> MGKYFGTDGVRGVANSELTPELAFKVGRFGGYVLTKDKQRPKVLIGRDTRISGHMLEGALVAGLLSIGAEVMRLGVISTPGVSYLTKAMDAEAGVMISASHNPVQDNGIKFFGGDGFKLSDEQEAEIERLMDEPEDKLPRPVGADLGLVNDYFEGGQKYLQFLKQTADEDFTGIHVALDCANGATSSLATHLFADLDADVSTMGTSPNGLNINDGVGSTHPEALSAFVKEKNADL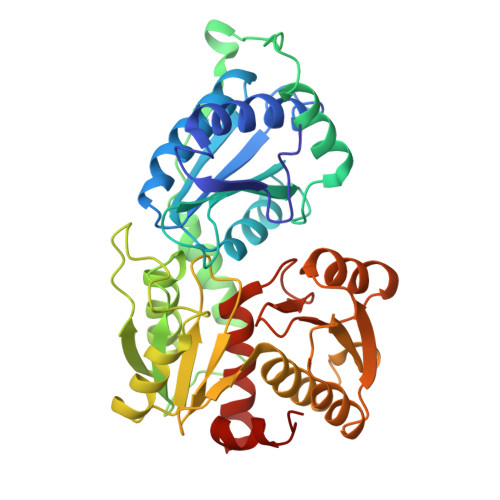GLAFDGDGDRLIAVDEKGNIVDGDQIMYICSKHLKSEGRLKDDTVVSTVMSNLGFYKALEKEGIKSVQTAVGDRYVVEAMKKDGYNVGGEQSGHLIFLDYNTTGDGLLSAIMLMNTLKATGKPLSELAAEMQKF>ETGKPSFVTFRGEPAEGFNHLVVDERTGHIYLGAVNRIYKLSSDLKVLVTHQTGPDEDNPKCYPPRIVQTCNEPLASTNNVNKMLLIDYKENRLIACGSLYQGICKLLRLEDLFKLGEPFHKKEHYLSGVNESGSVFGVIVSYSNFDDKLFIATAVDGKPEYFPTISSRKLTKNSEADGMFAYVFHDEFVASMIKIPSDTFTVIPDFDIYYVYGFSSGNFVYFLTLQPEMVSPPGSTTKEQVYTSKLVRLCKEDTAFNSYVEVPIGCERNGVEYRLLQAAYLSKAGAVLGRTLGVRPDDDLLFTVFSKGQKRKMKSLDESALCIFILKQINDRIKDRLQSCYRGEGTLDLAWLKVKDIPCSSALLTIDDNFCGLDMNAPLGVSEMVRGIPVFTEDRDRMTSVIAYVYKNHSLAFVGTKSGKLKKIRVDGPKGNALQYETVQVVDSGPVLRDMAFSKDHEQLYIMSERQLTRVPVESCGQYRSCGECLGSGDPHCGWCVLHNTCTRKERCERSREPRRFASEMKQCVRLTVHPNNISVSQYNVLLVLETYNVPELSAGVNCTFEDLSEMDGLVIGNQIQCYSPAAKEVPRIITENGDHHVVQLQLKSKETGMTFASTSFVFYNCSVHNSCLSCVESPYRCHWCKYRHVCTHDPNTCSFQEGRVKLPEDCPQLLRVDKILVPVEVIKPITLKAKNLPQPQSGQRGYECILNIQGIEQRVPALRFNSSSVQCQNTSYSYEGMEINNLPVELTVVWNGHFNIDNPAQNKVYLYKCGAMRESCGLCLKADPDFECGWCQSPGQCTLRQHCPAHESRWLELSGANSKCTNPRITEIIPVTGPREGGTKVTIRGENLGLEFRDIASHVKVAGVECSPLVDGYIPAEQIVCEMGEAKPSQHAGFVEICVAVCRPEFMARSSQLYYFMTLTLADLKPNRGPMSGGTQVTITGTNLNAGSNVVVMFGSQPCLFHRRSPSYIICNTTSSEEVLDMKVTVQVDRARIRQDLVFQYVEDPTIVRIEPEWSIVSGNTPIAVWGTHLDLIQNPQIRAKHGGKEHINICEVLNATEMTCQAPALALGPDHQSDLTER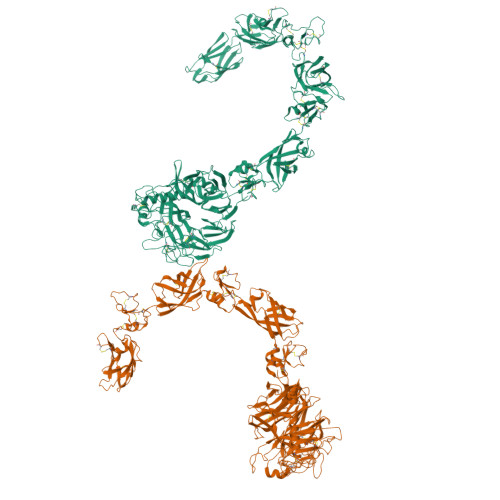PEEFGFILDNVQSLLILNKTNFTYYPNPVFEAFSPSGILELKPGTPIILKGKNLIPPVAGGNVKLNYTVLVGEKPCTVTVSDVQLLCESPNLIGRHKVMARVGGMEYSPGMVYIAPGRTKHHHHHH[2x]>[2x]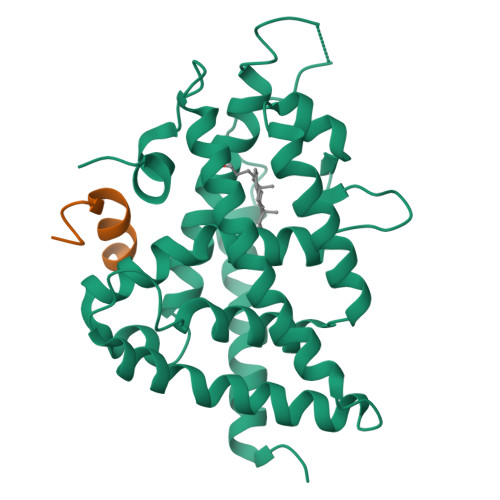GSEGEGVQLTAAQELMIQQLVAAQLQCNKRSFSDQPKVTPWPLGADPQSRDARQQRFAHFTELAIISVQEIVDFAKQVPGFLQLGREDQIALLKASTIEIMLLETARRYNHETECITFLKDFTYSKDDFHRAGLQVEFINPIFEFSRAMRRLGLDDAEYALLIAINIFSADRPNVQEPGRVEALQQPYVEALLSYTRIKRPQDQLRFPRMLMKLVSLRTLSSVHSEQVFALRLQDKKLPPLLSEIWDVHE;>CPSSHSSLTERHKILHRLLQEGSPS[2x]>NNPSAAVVVSSRWNPTPEQLRALEELYRRGTRTPSAEQIQQITAQLRKFGKIEGKNVFYWFQNHKARERQKRRRQMESAA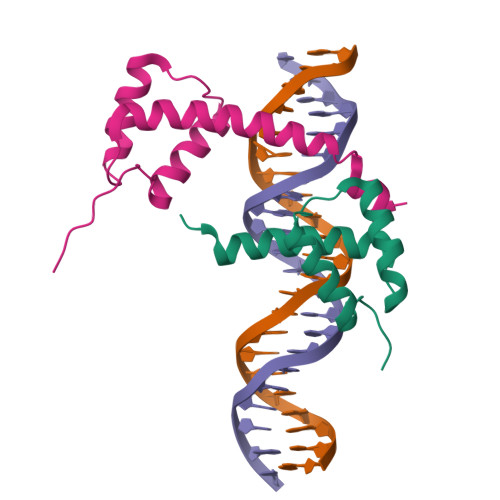AEFDSAIEKKDLGASRTVFEVEHTKN[2x]>MEEGFRDRAAFIRGAKDIAKEVKKHAAKKVVKGLDRVQDEYSRRSYSRFEEEDDDDDFPAPSDGYYRGEGTQDEEEGGASSDATEGHDEDDEIYEGEYQGIPRAESGGKGERMADGAPLAGVRGGLSDGEGPPGGRGEAQRRKEREELAQQYEAILRECGHGRFQWTLYFVLGLALMADGVEVFVVGFVLPSAEKDMCLSDSNKGMLGLIVYLGMMVGAFLWGGLADRLGRRQCLLISLSVNSVFAFFSSFVQGYGTFLFCRLLSGVGIGGSIPIVFSYFSEFLAQEKRGEHLSWLCMFWMIGGVYAAAMAWAIIPHYGWSFQMGSAYQFHSWRVFVLVCAFPSVFAIGALTTQPESPRFFLENGKHDEAWMVLKQVHDTNMRAKGHPERVFSVTHIKTIHQEDELIEIQSDTGTWYQRWGVRALSLGGQVWGNFLSCFGPEYRRITLMMMGVWFTMSFSYYGLTVWFPDMIRHLQAVDYASRTKVFPGERVEHVTFNFTLENQIHRGGQYFNDKFIGLRLKSVSFEDSLFEECYFEDVTSSNTFFRNCTFINTVFYNTDLFEYKFVNSRLINSTFLHNKEGCPLDVTGTGEGAYM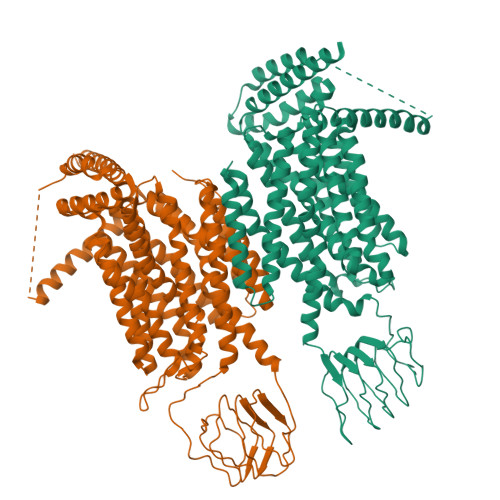VYFVSFLGTLAVLPGNIVSALLMDKIGRLRMLAGSSVMSCVSCFFLSFGNSESAMIALLCLFGGVSIASWNALDVLTVELYPSDKRTTAFGFLNALCKLAAVLGISIFTSFVGITKAAPILFASAALALGSSLALKLPSRLEEELRRRTEPGSLEVLFQ[2x]N-(piperidin-4-yl)-6-(trifluoromethyl)pyrimidin-4-amine | C10 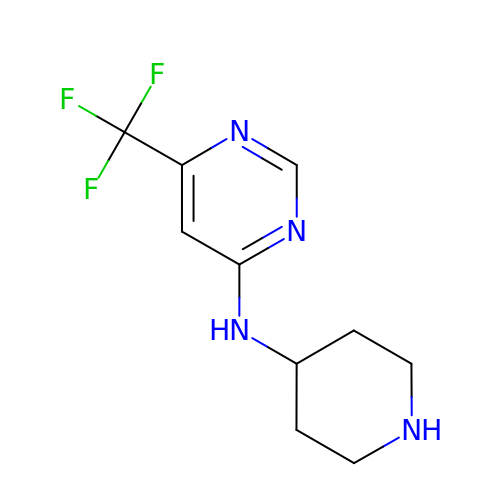H13 F3 N4 | GRSDOXXGQOHABE-UHFFFAOYSA-N> GAAPDAVMVFARQGDKGSVSVGDKHFRTQAFKVRLVNAAKSEISLKN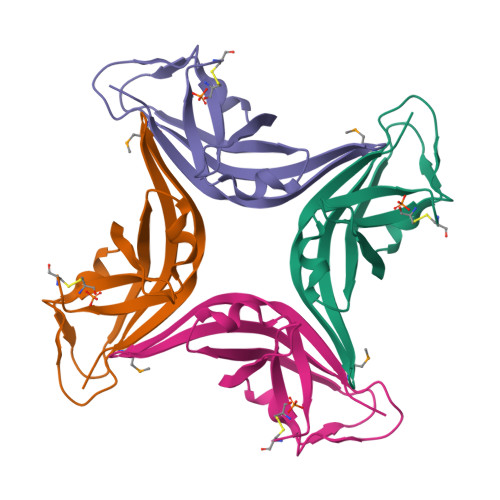SCLVAQSAAGQSFRLDTVDEELTADTLKPGASVEGDAIFASEDDAVYGASLVRLSDRCK>MFRILTINPGSTSTKLSIFEDERMVKMQNFSHSPDELGRFQKILDQLEFREKIARQFVEETGYSLSSFSAFVSRGGLLDPIPGGVYLVDGLMIKTLKSGKNGEHASNLGAIIAHRFSSETGVPAYVVDPVVVDEMEDVARVSGHPNYQRKSIFHALNQKTVAKEVARMMNKRYEEMNLVVAHMGGGISIAAHRKGRVIDVNNALDGDGPFTPERSGTLPLTQLVDLCFSGKFTYEEMKKRIVGNGGLVAYLGTSDAREVVRRIKQGDEWAKRVYRAMAYQIAKWIGKMAAVLKGEVDFIVLTGGLAHEKEFLVPWITKRVSFIAPVLVFPG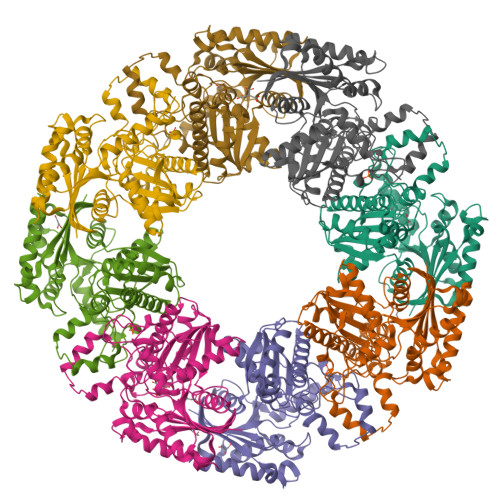SNEEKALALSALRVLRGEEKPKNYSEESRRWRERYDSYLDGILR[8x]> MKLTPKEQEKFLLYYAGEVARKRKEEGLKLNQPEAIAYISAHIMDEARRGKKTVAQLMEECVHFLKKDEVMPGV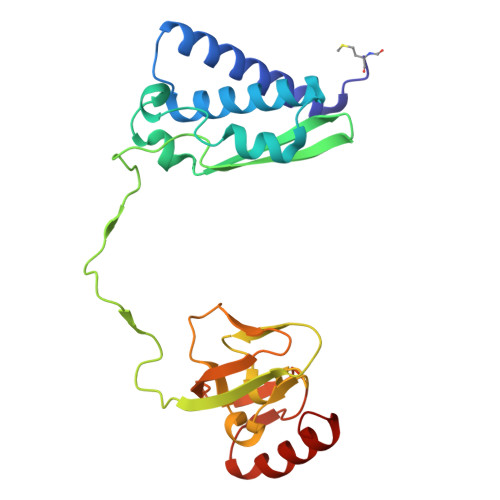GNMVPDLGVEANFPDGTKLVTVNWPIEPDDFKAGEIKFASDKDIELNAGKEITELKVTNKGPKSLHVGSHFHFFEANRALEFDREKAYGKRLDIPSGNTLRIGAGETKTVHLIPIGGSKKIIGMNGLLNGIADDLHKQKALEKAKHHGFIK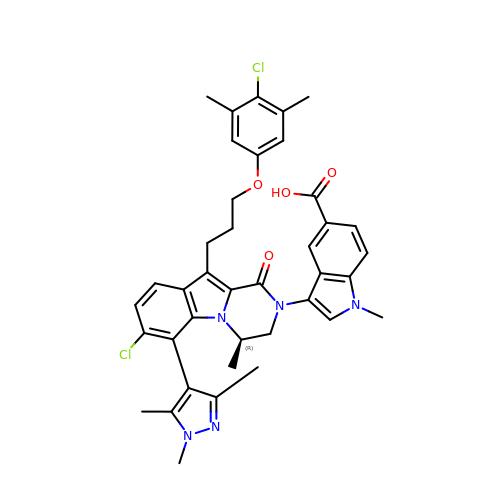3-[(4R)-7-chloro-10-[3-(4-chloro-3,5-dimethylphenoxy)propyl]-4-methyl-1-oxo-6-(1,3,5-trimethyl-1H-pyrazol-4-yl)-3,4-dihydropyrazino[1,2-a]indol-2(1H)-yl]-1-methyl-1H-indole-5-carboxylic acid | C39 H39 Cl2 N5 O4 | BSAYHBZFNXDOIJ-JOCHJYFZSA-N>MAGKAHRLS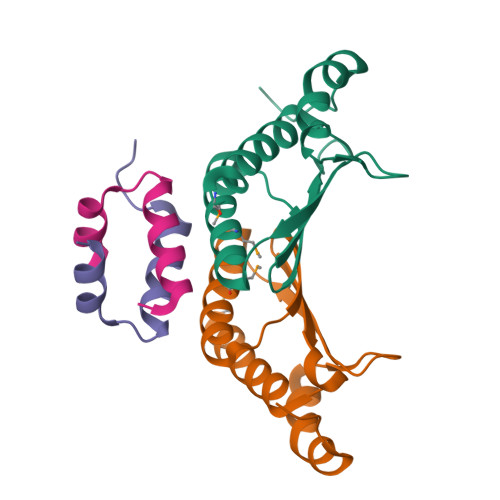AEERDQLLPNLRAVGWNELEGRDAIFKQFHFKDFNRAFGFMTRVALQAEKLDHHPEWFNVYNKVHITLSTHECAGLSERDINLASFIEQVAVSMT[4x];>[4x]MVSKLSQLQTELLAALLESGLSKEALIQALGE>[2x]MAKNRRDRNSWGGFSEKTYEWSSEEEEPVKKAGPVQVLIVKDDHSFELDETALNRILLSEAVRDKEVVAVSVAGAFRKGKSFLMDFMLRYMYNQESVDWVGDYNEPLTGFSWRGGSERETTGIQIWSEIFLINKPDGKKVAVLLMDTQGTFDSQSTLRDSATVFAL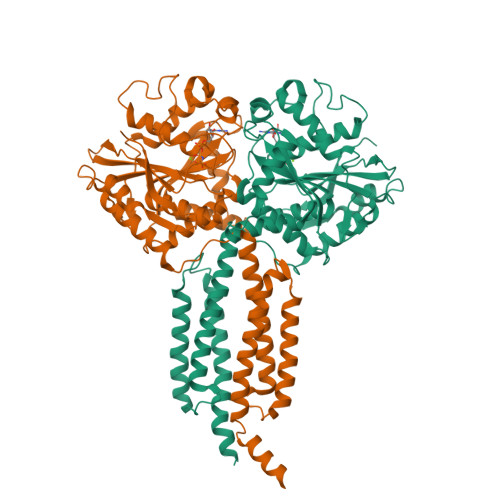STMISSIQVYNLSQNVQEDDLQHLQLFTEYGRLAMEETFLKPFQSLIFLVRDWSFPYEFSYGADGGAKFLEKRLKVSGNQHEELQNVRKHIHSCFTNISCFLLPHPGLKVATNPNFDGKLKEIDDEFIKNLKILIPWLLSPESLDIKEINGNKITCRGLVEYFKAYIKIYQGEELPHPKSMLQATAEANNLAAVATAKDTYNKKMEEICGGDKPFLAPNDLQTKHLQLKEESVKLFRGVKKMGGEEFSRRYLQQLESEIDELYIQYIKHNDSKNIFHAARAAALEHHHHHH>[3x]MTYGGRDQQYNKTNYKSRGGDFRGGRNSDRNSYNDRPQGGNYRGGFGGRSNYNQPQELIKPNWDEELPKLPTFEKNFYVEHESVRDRSDSEIAQFRKENEMTISGHDIPKPITTFDEAGFPDYVLNEVKAEGFDKPTGIQCQGWPMALSGRDMVGIAATGSGKTLSYCLPGIVHINAQPLLAPGDGPIVLVLAPTRELAVQIQTECSKFGHSSRIRNTCVYGGVPKSQQIRDLSRGSEIVIATPGRLIDMLEIGKTNLKRVTYLVLDEADRMLDMGFEPQIRKIVDQIRPDRQTLMWSATWPKEVKQLAADYLNDPIQVQVGSLELSASHNITQIVEVVSDFEKRDRLNKYLETASQDNEYKTLIFASTKRMCDDITKYLREDGWPALAIHGDKDQRERDWVLQEFRNGRSPIMVATDVAARGIDVKGINYVINYDMPGNIEDYVHRIGRTGRAGATGTAISFFTEQNKGLGAKLISIMREANQNIPPELLKYDRRSYGGGHPRYGGGRGGRGGYGRRGGYGGGRGGYGGNRQRDGGWGNRGRSNY

Human DDX5 and its yeast ortholog Dbp2 are ATP-dependent RNA helicases that play a key role in normal cell processes, cancer development, and viral infection. Similar to other DEAD-box proteins, DDX5/Dbp2 is composed of two RecA-like domains that include 11 conserved motifs. The helicase core of Dbp2 consists of two RecA-like domains (RecA1: aa 101–319; RecA2: aa 332–465), an NTE (aa 53–100), a CTE (aa 466–496), and a linker (aa 320–331). Here, we report the first X-ray crystal structures of the Dbp2 helicase core alone and in complex with ADP at 3.22 Å and 3.05 Å resolutions, respectively.

The Dbp2 catalytic core apo (Dbp2-apo) crystallized in space group C121 with 2.5 molecules in the asymmetric unit: two molecules (aa 57–496) in nearly identical conformation (rmsd 1.11 Å) and a half molecule (aa 57–326). This molecule fragment composed of NTE-RecA1 is likely generated by the limited proteolysis of the linker between the RecA1 and RecA2 domains. In the crystal structure of Dbp2-apo, two RecA-like domains adopted an open state, with the NTE subdomain located on the exterior surface of RecA1 and the CTE subdomain inserted between two RecA-like domains. To estimate the position and intrinsic mobility of the two RecA-like domains, we calculated the distance between the centers of mass of the RecA1 and RecA2. This distance was 42.9 Å in the open state, showing that the two domains were far apart, as shown in Figure 2B. In the Dbp2-apo structure, the RecA1 and RecA2 domains are restrained by the linker and CTE subdomains. The RecA1, RecA2, NTE, CTE subdomains, and linker form an interaction network, stabilizing the conformation. In the structure of Dbp2-apo, the CTE consists of an α-helix and a disordered loop that inserts into the cleft of the helicase core. Residues R495 and R496 of the CTE form five hydrogen bonds with V128, E131, and T137 of the Q motif in the RecA1 domain (black box). We solved the first crystal structure of Dbp2 to date, illustrating that the protein is rigid and in an open state. In contrast, the CTE has two conformations: one in which Dbp2-apo is wedged between the helicase core and one in which the addition of ADP induces it to move out of the way of the ATP binding site.> MDINELIIGAQSADKHTREVAETQLLQWCDSDASQVFKALANVALQHEASLESRQFALLSLRKLITMYWSPGFESYRSTSNVEIDVKDFIREVLLKLCLNDNENTKIKNGASYCIVQISAVDFPDQWPQLLTVIYDAISHQHSLNAMSLLNEIYDDVVSEEMFFEGGIGLATMEIVFKVLNTETSTLIAKIAALKLLKACLLQMSSHNEYDEASRKSFVSQCLATSLQILGQLLTLNFGNVDVISQLKFKSIIYENLVFIKNDFSRKHFSSELQKQFKIMAIQDLENVTHINANVETTESEPLLETVHDCSIYIVEFLTSVCTLQFSVEEMNKIITSLTILCQLSSETREIWTSDFNTFVSKETGLAASYNVRDQANEFFTSLPNPQLSLIFKVVSNDIEHSTCNYSTLESLLYLLQCILLNDDEITGENIDQSLQILIKTLENILVSQEIPELILARAILTIPRVLDKFIDALPDIKPLTSAFLAKSLNLALKSDKELIKSATLIAFTYYCYFAELDSVLGPEVCSETQEKVIRIINQVSSDAEEDTNGALMEVLSQVISYNPKEPHSRKEILQAEFHLVFTISSEDPANVQVVVQSQECLEKLLDNINMDNYKNYIELCLPSFINVLDSNNANNYRYSPLLSLVLEFITVFLKKKPNDGFLPDEINQYLFEPLAK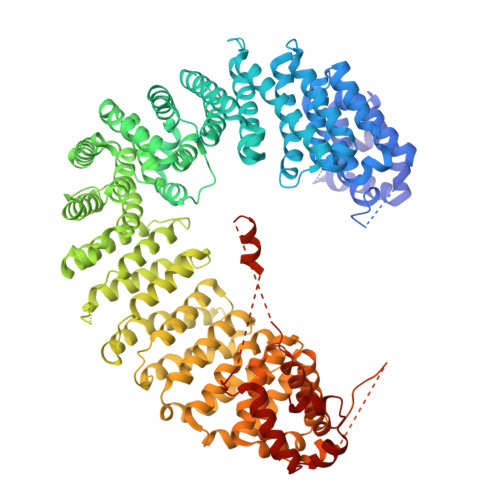VLAFSTEDETLQLATEAFSYLIFNTDTRAMEPRLMDIMKVLERLLSLEVSDSAAMNVGPLVVAIFTRFSKEIQPLIGRILEAVVVRLIKTQNISTEQNLLSVLCFLTCNDPKQTVDFLSSFQIDNTDALTLVMRKWIEAFEVIRGEKRIKENIVALSNLFFLNDKRLQKVVVNGNLIPYEGDLIITRSMAKKMPDRYVQVPLYTKIIKLFVSELSFQSKQPNPEQLITSDIKQEVVNANKDDDNDDWEDVDDVLDYDKLKEYIDDDVDEEADDDSDDITGLMDVKESVVQLLVRFFKEVASKDVSGFHCIYETLSDSERKVLSEALL>[4x]MLPVELVRHDVKKTDETSQVELMLQVDPDLFWFNGHFTGQPLLPGVAQLDWVMHYAT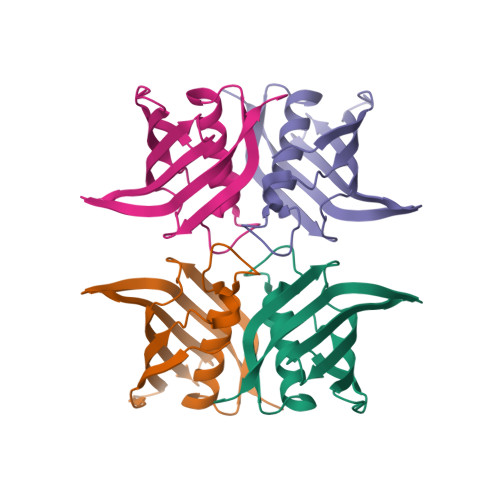TVLAQGWTFLSIENIKFQQPILPGKTLRLVLIWHAGKQSLTFSYSILEGDTERTASSGKIKLTPIMEDNPCQ Echovirus 3 (E3), a serotype of HEV-B, first isolated in 1953, leads to highly contagious and severe diseases in humans, such as aseptic meningitis, myocarditis, and anicteric hepatitis. In line with many other HEV-Bs, E3 utilizes CD55 for viral attachment and FcRn for viral uncoating, gaining efficient entry into the host cells. Following rounds of purifications and analyses, three types of particles were identified, one containing significant amounts of viral RNA characterized as mature virus (or full particle, F-particle) and the other two being empty inside with substantially different sizes defined as expanded and compact empty particles (EE- and EC-particles). A number of key structural elements, including the VP1 BC, DE loops and C-terminus, the VP2 EF loop and VP3 EF, GH loops, contribute to the serotype-specific antigenic sites and construct the “canyon”, where many HEV receptors often bind.

Cryo-electron microscopic (cryo-EM) structures of the three types of particles: F-particle (~ 64%), EC-particle (~ 3%), and EE-particle (~ 33%) were reconstructed to 3.2 Å, 3.8 Å, and 3.1 Å resolution, respectively. The external surfaces of the F- and EC-particles with a diameter of ~ 325 Å are indistinguishable, apart from some disorder on the inside of the EC-particle, including N-termini of VP1 and VP0. Superimposition of the asymmetric units (protomers) verifies the similarity in capsid structures of the F- and EC-particles and reveals substantially conformational differences between F- and EE-particles in several exposed loops, such as VP1 BC, DE, EF and HI loops, VP3 EF and GH loops. Remarkably, most of these loops are key determinants for immunogenicity in HEVs, indicating that EC-particle, rather than EE-particle, has more potential as candidates for the development of a vaccine. Notably, VP1 C-terminus, appearing to be the most divergent in sequence among the four subgroups in HEV-Bs, is largely disordered in the native virus structures (F-, EC-, and EE-particles), indicative of a cryptic immunogenic site, akin to the VP1 GH loop in foot-and-mouth disease virus (FMDV). In summary, the atomic structures of E3 mature virion and the two types of empty particles reveal serotype-specific structural features between the subgroups within HEV-Bs and underline the potential of E3 F- or EC-particles as ideal vaccine candidates.

> GDVEEAIDRAVARVADTMPTGPRNTESVPALTAVETGHTSQVVPGDTMQTRHVKNYHSRTESSIENFLCRAACVYIATYKSAGGTPTERYASWRINTRQMVQLRRKFELFTYLRFDMEITFVITSTQDPGTQLAQDMPVLTHQIMYIPPGGPVPNSATDFAWQSSTNPSIFWTEGCAPARMSVPFISIGNAYSNFYDGWSHFTQEGVYGFNSLNNMGHIYVRHVNEQSLGVSTSTLRVYFKPKHVRAWVPRPPRLSPYVKSSNVNFKPTAVTTERKDINDVGTLRPVGYTNH;> GAQVSTQKTGAHETSLTASGNSTIHYTNINYYKDAASNSANRQDFTQDPSKFTEPMKDVMIKSLPALNSPTVEECGFSDRVRSITLGNSTITTQECANVVVGYGVWPSYLQDNEATAEDQPTQPDVATCRFYTLDSIQWQKESDGWWWKFPEALKNMGLFGQNMEYHYLGRSGYTIHVQCNASKFHQGCLLVVCVPEAEMGCSDVEREVVAASLSSEDTAKSFSRTESNGQHTVQTVVYNAGMGVGVGNLTIFPHQWINLRTNNSATIVMPYINSVPMDNMFRHYNFTLMIIPFAKLEYTEQASNYVPITVTVAPMCAEYNGLRLASHQ;> GLPTMLTPGSNQFLTSDDFQSPSAMPQFDVTPEMKIPGEVHNLMEIAEVDSVVPVNNTKENINSMEAYRIPVTGGDQLHTQVFGFQMQPGLNSVFKRTLLGEILNYYAHWSGSVKLTFVFCGSAMATGKFLLAYSPPGASPPQNRKQAMLGTHVIWDVGLQSSCVLCIPWISQTHYRLVQQDEYTSAGYVTCWYQTGLIVPPGAPPSCTILCFASACNDFSVRNLRDTPFIEQTQLLQ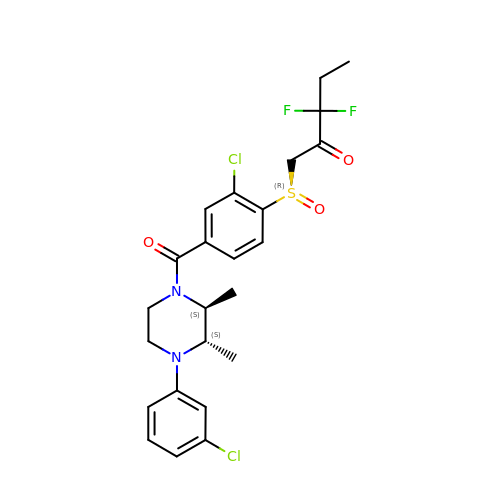1-[(~{R})-[2-chloranyl-4-[(2~{S},3~{S})-4-(3-chlorophenyl)-2,3-dimethyl-piperazin-1-yl]carbonyl-phenyl]sulfinyl]-3,3-bis(fluoranyl)pentan-2-one | C24 H26 Cl2 F2 N2 O3 S | WYHRZGBTLDYJGW-GLVLYPABSA-N>MHRTYSLRNSRAPTASQLQNPPPPPSTTKGRFFGKGGLAYSFRRSAAGAFGPELSRKLSQLVKIEKNVLRSMELTANERRDAAKQLSIWGLENDDDVSDITDKLGVLIYEVSELDDQFIDRYDQYRLTLKSIRDIEGSVQPSRDRKDKITDKIAYLKYKDPQSPKIEVLEQELVRAEAESLVAEAQLSNITRSKLRAAFNYQFDSIIEHSEKIALIAGYGKALLELLDDSPVTPGETRPAYDGYEASKQIIIDAESALNEWTLDSAQVKPT[2x]

The yeast eisosome, composed of the BAR-domain proteins Pil1 and Lsp1 (hereafter, Pil1/Lsp1), scaffolds a membrane compartment that senses and responds to mechanical stress by flattening and releasing sequestered factors. MCC–eisosomes are relatively stable, and have been implicated in sensing and responding to plasma membrane stress: various stimuli, including hypo-osmotic shock, heat shock and mechanical pressure, cause eisosomes to flatten and release sequestered proteins to affect signalling or transport functions. Here we isolated near-native eisosomes as helical tubules made up of a lattice of Pil1/Lsp1 bound to plasma membrane lipids, and solved their structures by helical reconstruction.

Three-dimensional variability analysis of the native-source eisosomes revealed a dynamic stretching of the Pil1/Lsp1 lattice that affects the sequestration of these lipids. We also saw that changes in the shape and size of the bound lipid density were synchronized with the stretching of the Nt contact sites in the visualization of the 3D variability. To characterize the relationship between the Nt stretching and the changes in the lipid density, we extracted ten sets of non-overlapping particles along this variability dimension for further refinement, which allowed us to compare the most compact and most stretched lattice classes. Particles from every tubule diameter are distributed across all ten classes; however, particles from small-diameter tubules are overrepresented in the more compact classes, whereas those from large-diameter tubules are overrepresented in more stretched classes. This suggests that the flexibility we observe arises from the protein lattice stretching to accommodate larger diameters of tubules. Although the most compressed protein lattice class retained the pattern of membrane voids beneath the AH, indicating sterol binding, this pattern was gradually lost in the intermediate classes and was blurred in the most stretched protein lattice class, despite its slightly higher resolution. In our native-source structures, we see that Pil1 lattice stretching is correlated with a mobilization of PI(4,5)P2 and PS and a loss of the sterol patterning within the cytoplasmic leaflet, which implies an increased mobility of all of the lipids within the MCC–eisosome.>MSVIKPEMKIKLRMEGAVNGHKFVIEGEGIGKPYEGTQTLDLTVKEGAPLPFSYDILTPAFMYGNRAFVKYPKDIPDYFKQAFPEGYSWERSMTYEDQGICIATSDITMEGDCFFYKIRFDGTNFPPNGPVMQKKTLKWEPSTEKMYVRDGVLKGDVNMALLLEGGGHYRCDFKTTYKAKKDVRLPDAHEVDQRIEILSHDKDYNKVRLYEHAEARYSMLPSQAKASGKP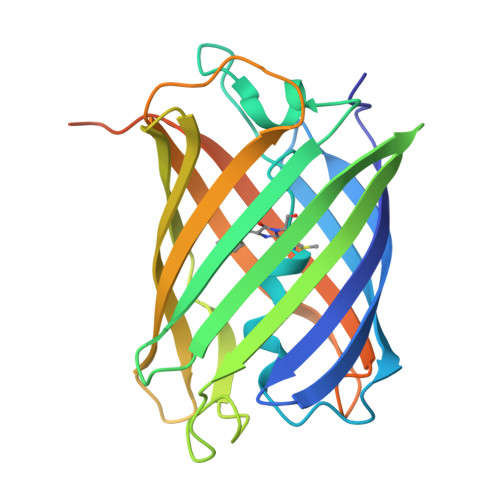IPNPLLGLDSTHHHHHH[4x]>[2x]GSSPVRLAPEREFIKSLMAIGKRLATLPTKEQK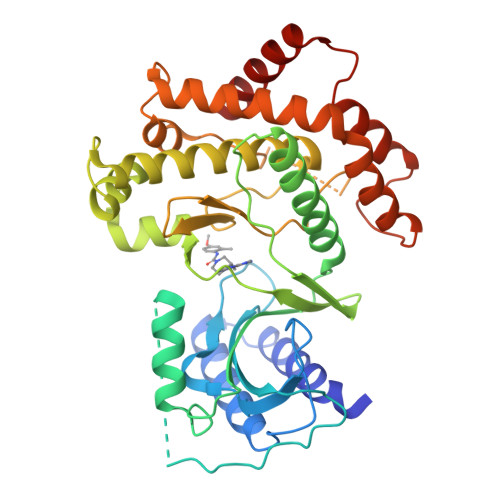TQRLISELSLLNHKLPARVWLPTAGFDHHVVRVPHTQAVVLNSKDKAPYLIYVEVLECENFDTTSVPARIPENRIRSTRSDSGDGSALKEPWQEKVRRIREGSPYGHLPNWRLLSVIVKCGDDLRQELLAFQVLKQLQSIWEQERVPLWIKPYKILVISADSGMIEPVVNAVSIHQVKKQSQLSLLDYFLQEHGSYTTEAFLSAQRNFVQSCAGYCLVCYLLQVKDRHNGNILLDAEGHIIHIDFGFILSSSPRNLGFETSAFKLTTEFVDVMGGLDGDMFNYYKMLMLQGLIAARKHMDKVVQIVEIMQQGSQLPCFHGSSTIRNLKERFHMSMTEEQLQLLVEQMVDGSMR>[2x]NDDKLYRADSRPPDEIKQSGGLMP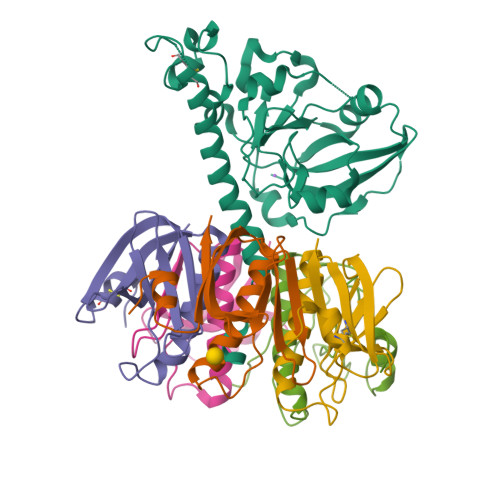RGQSEYFDRGTQMNINLYDHARGTQTGFVRHDDGYVSTSISLRSAHLVGQTILSGHSTYYIYVIATAPNMFNVNDVLGAYSPHPDEQEVSALGGIPYSQIYGWYRVHFGVLDEQLHRNRGYRDRYYSNLDIAPAADGYGLAGFPPEHRAWREEPWIHHAPPGCGNAPRSSMSNTCDEKTQSLGVKFLDEYQSKVKRQIFSGYQSDIDTHNRIKDEL;>TPQNITDLCAEYHNTQIHTLNDKIFSYTESLAGKREMAIITFKNGATFQVEVPGSQHIDSQKKAIERMKDTLRIAYLTEAKVEKLCVWNNKTPHAIAAISMAN[10x]>MAEETIFSKIIRREIPSDIVYQDDLVTAFRDISPQAPTHILIIPNILIPTVNDVSAEHEQALG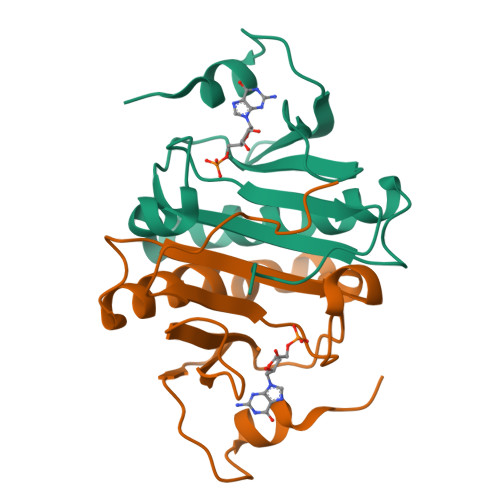RMITVAAKIAEQEGIAEDGYRLIMNTNRHGGQEVYHIAMHLLGGRPLGPMLAHKGL[4x]> MLSVRTPLATIADQQQLQLSPLKRLTLADKENTPPTLSSTRVLASKAARRIFQDSAELESKAPTNPSVEDEPLLRENPRRFVVFPIEYHDIWQMYKKAEASFWTAEEVDLSKDIQHWEALKPDERHFISHVLAFFAASDGIVNENLVERFSQEVQVTEARCFYGFQIAMENIHSE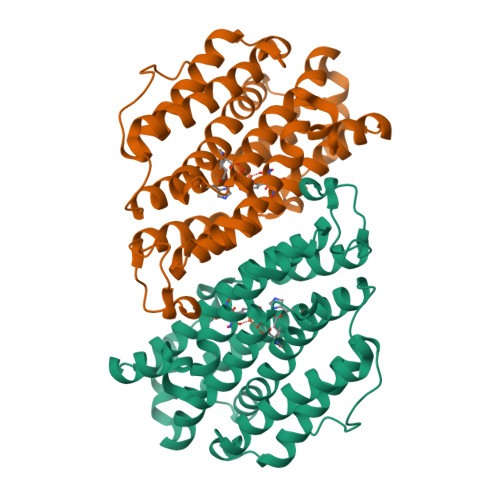MYSLLIDTYIKDPKEREYLFNAIETMPCVKKKADWALRWIGDKEATYGERVVAFAAVEGIFFSGSFASIFWLKKRGLMPGLTFSNELISRDEGLHCDFACLMFKHLVHKPAEQRVREIITNAVRIEQEFLTEALPVKLIGMNCTLMKQYIEFVADRLMLELGFNKIFRVENPFDFMENISLEGKTNFFEKRVGEYQRMGVMSNSTENSFTLDADF>[2x]GSPSTRDYEIQRERIELGRCIGEGQFGDVHQGIYMSPENPALAVAIKTCKNCTSDSVRE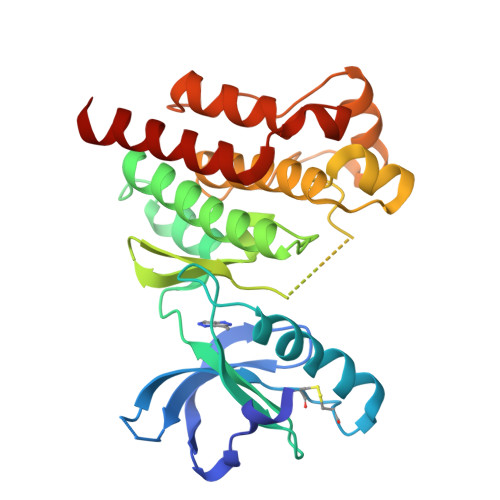KFLQEALTMRQFDHPHIVKLIGVITENPVWIIMELCTLGELRSFLQVRKYSLDLASLILYAYQLSTALAYLESKRFVHRDIAARNVLVSSNDCVKLGDFGLSRYMEDSTYYKASKGKLPIKWMAPESINFRRFTSASDVWMFGVCMWEILMHGVKPFQGVKNNDVIGRIENGERLPMPPNCPPTLYSLMTKCWAYDPSRRPRFTELKAQLSTILEEEKAQ In this study, we have biochemically and structurally characterized the NADP⁺-dependent EhME, identifying its role in metronidazole (Mtz) activation. Malic enzyme (ME) catalyzes the conversion of malate to pyruvate through a two-step reaction. Complementation assays and E-tests demonstrate that overexpression of EhME in bacterial cells increases their susceptibility to Mtz. Upon incubation of rEhME with Eh cells or human enteric cells (Caco-2 and HT29), it was evident that EhME binds efficiently to both.

The crystal structure of EhME was determined at a resolution of 2.2 Å using the platinum single isomorphous replacement with anomalous scattering (SIRAS) method. The crystal belongs to space group P43212, with two nearly identical monomers in the asymmetric unit, exhibiting an RMSD of 0.35 Å across 3581 atoms. The monomer structure is organized into five distinct domains. Unlike most metazoan malic enzymes, which are typically homotetramers, EhME exists strictly as a dimer, with the two protomers deeply entangled. The N- and C-terminal regions of each protomer come into close proximity, forming a loop-like structure that secures a portion of the second protomer, resulting in a knot-like arrangement. The catalytic triad of EhME is composed of Tyr65, Lys120, and Asp193. Due to the knotted structure of EhME, two monomers engage in inter-monomer swapping of these motifs, contributing to the formation of each other’s active site. In the EhME structure, a water molecule occupies the putative metal-binding site, bridging hydrogen bonding interactions between the protein and a glycerol molecule. Notably, a sulfate molecule in the crystal structure mimics the 2′-ribose phosphate of NADP⁺ at its binding site. In EhME, the knotted structure appears to enhance structural resilience, allowing the enzyme to withstand mechanical and environmental stresses associated with its secretion.

>[2x]MAQLKADLSNLEECLPSTLSQEQRAVAKTQFYKELAEKVHKFYKGKIQIMPKCTLAGFNWFNAYYTPGVSRISTNIRDNNDSSLFYSLRGNFVGVVSDSTRVLGDGDVTPPGGLGVMEGKALLMKYLGGIDAVPICIDSKNKEGKNDPDAVIEFVQRIQHTFGAINLEDISQPNCYKILDVLRESCDIPVWHDDQQGTASVTLAGLLNALKLVKKDIHECRMVFIGAGSSNTTCLRLIVTAGADPKKIVMFDSKGSLHNGREDIKKDTRFYRKWEICETTNPSKFGSIAEACVGADVLISLSTPGPGVVKAEWIKSMGEKPIVFCCANPVPEIYPYEAKEAGAYIVATGRGDFPNQVNNSVGFPGILKGALIVRARKITDNMAIAASRALAEFAEKRGINPDNIIGTMDEPGIFPKEAADVAMQAIKDGVARVTDLTWQQVYDIAEHDIKEARESAQLLQDSKHIVDFPQETLNECLAYAINKVTGK> PISPIETVPVKLKPGMDGPKVKQWPLTEEKIKALVEICTEMEKEGKISKIGPENPYNTPVFAIKKKDSTKWRKLVDFRELNKRTQDFWEVQLGIPHPAGLKKKKSVTVLDVGDAYFSVPLDEDFRKYTAFTIPSINNETPGIRYQYNVLPQGWKGSPAIFQSSMTKILEPFKKQNPDIVIYQYMDDLYVGSDLEIGQHRTKIEELRQHLLRWGLTTPDKKHQKEPPFLWMGYELHPDKWTVQPIVLPEKDSWTVNDIQKLVGKLNWASQIYPGIKVRQLCKLLRGTKALTEVIPLTEEAELELAENREILKEPVHGVYYDPSKDLIAEIQKQGQGQWTYQIYQE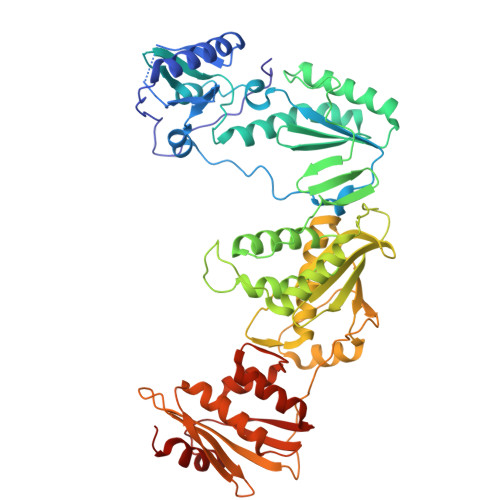PFKNLKTGKYARMRGAHTNDVKQLTEAVQKITTESIVIWGKTPKFKLPIQKETWETWWTEYWQATWIPEWEFVNTPPLVKLWYQLEKEPIVGAETFYVDGAANRETKLGKAGYVTNKGRQKVVPLTNTTNQKTQLQAIYLALQDSGLEVNIVTDSQYALGIIQAQPDKSESELVNQIIEQLIKKEKVYLAWVPAHKGIGGNEQVDKLVSAGIR> PFVNKQFNYKDPVNGVDIAYIKIPNAGQMQPVKAFKIHNKIWVIPERDTFTNPEEGDLNPPPEAKQVPVSYYDSTYLSTDNEKDNYLKGVTKLFERIYSTDLGRMLLTSIVRGIPFWGGSTIDTELKVIDTNCINVIQPDGSYRSEELNLVIIGPSADIIQFECKSFGHEVLNLTRNGYGSTQYIRFSPDFTFGFEESLEVDTNPLLGAGKFATDPAVTLAHQLIHAGHRLYGIAINPNRVFKVNTNAYYEMSGLEVSFEELRTFGGHDAKFIDSLQENEFRLYYYNKFKDIASTLNKAKSIVGTTASLQYMKNVFKEKYLLSEDTSGKFSVDKLKFDKLYKMLTEIYTEDNFVKFFKVLNRKTFLNFDKAVFKINIVPKVNYTIYDGFNLRNTNLAANFNGQNTEINNMNFTKLKNFTPLVPR;> MDENLEQVSGII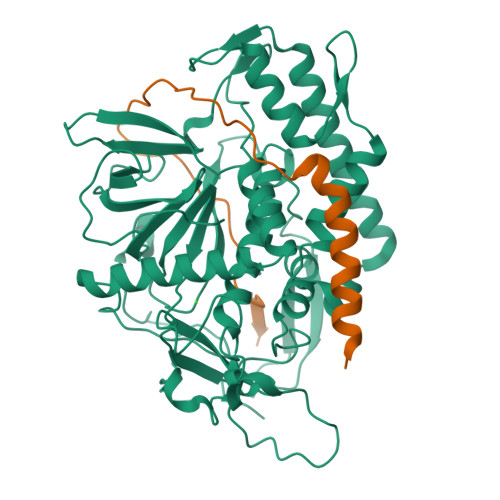GNLRHMALDMGNEIDTQNRQIDRIMEKADSNKTRIDEANQRATKMLG AMINOETHANOLPYROPHOSPHATE 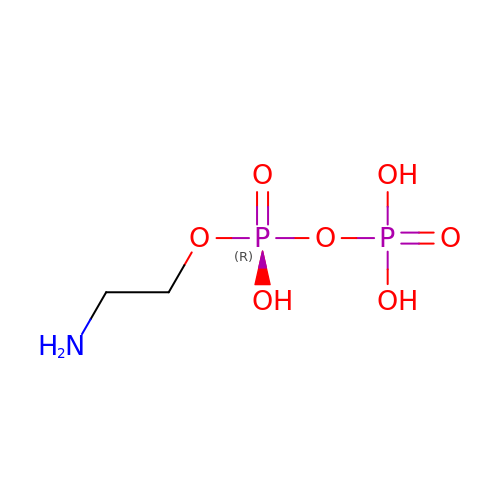| C2 H9 N O7 P2 | VOBNSQKMDIOJTQ-UHFFFAOYSA-N N-{5-[4-(2-amino-4-oxo-3,4-dihydrothieno[2,3-d]pyrimidin-6-yl)butyl]thiophene-2-carbonyl}-L-glutamic acid | C20 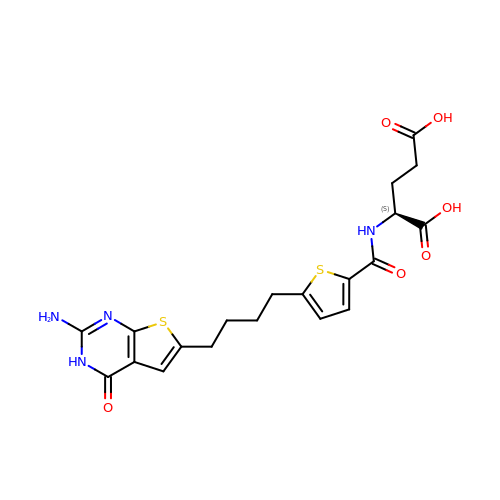H22 N4 O6 S2 | IFTGJDSAOAUHRL-ZDUSSCGKSA-N> GKLKKKGYLRIVTTQGSLNIELHADMAPRACDSFLRLCAVKYFDDTIFHRCIRNFMIQGGRAELRQPSKKKEVQQSPRSISGFPGGAPFEDEFDNRLVHQGIGVLSMANDGKHSNLSEFFITFKSCEHLNNKHTIFGRVVGGLDV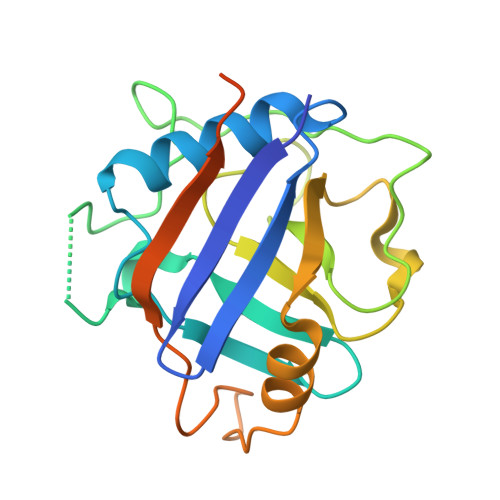LRQWEKLETDKKDKPLKPPKVEEIIVFKNPFEDARKEMEDEKREEEEKEKKKLENA2-amino-8-bromo-9-[(2R,4aR,6R,7R,7aS)-2,7-dihydroxy-2-oxotetrahydro-2H,4H-2lambda~5~-furo[3,2-d][1,3,2]dioxaphosphinin-6-yl]-1,9-dihydro-6H-purin-6-one | C10 H11 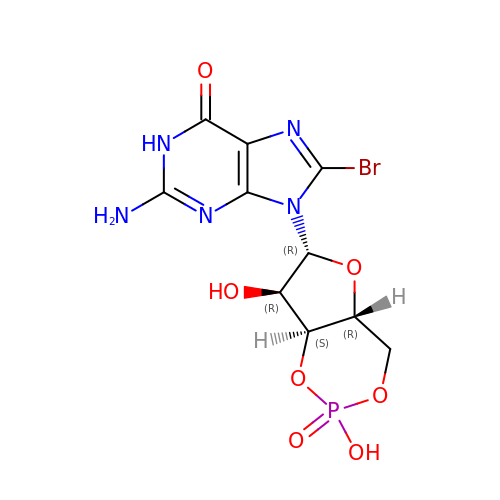Br N5 O7 P | YUFCOOWNNHGGOD-UMMCILCDSA-N>MIIKDILRENQDFRFRDLSDLKHSPKLCIITCMDSRLIDLLERALGIGRGDAKVIKNAGNIV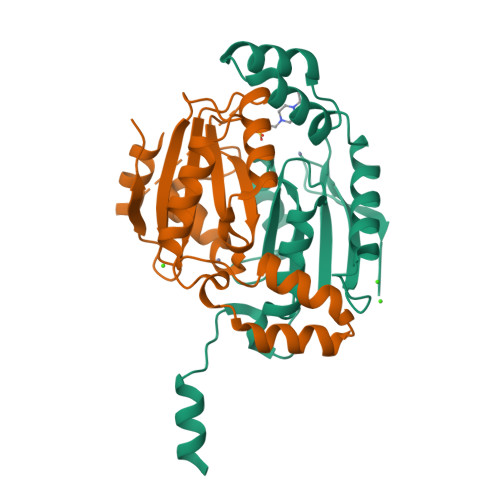DDGVIRSAAVAIYALGDNEIIIVGHTDCGMARLDEDLIVSRMRELGVEEEVIENFSIDVLNPVGDEEENVIEGVKRLKSSPLIPESIGVHGLIIDINTGRLKPLYLDE[6x]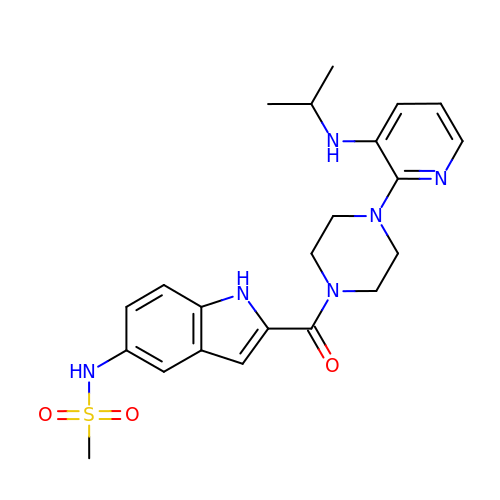(1-(5-METHANSULPHONAMIDO-1H-INDOL-2-YL-CARBONYL)4-[METHYLAMINO)PYRIDINYL]PIPERAZINE | C22 H28 N6 O3 S | WHBIGIKBNXZKFE-UHFFFAOYSA-N> MAFSAGAESLLHQAREIQDEELRRFCSRVTKLLQEAPGPATVDALQRLFLIVSATKYPRRLEKMCVDLLQTTLCLPASPEQLQVLCAAILREMSPFNDLALSCDHTPNTRQLSLVASVLLAQGDRKGEIRCVSQRIFKILENRQPEGPSVRPLLPILSKVIGLAPGILMEDQTNLLSKRLVDWLRYASIQQGLPYSGGFFSTPRTRQPGPITEVDGAVASDFFTVLSTGQHFTEDQWVNMQAFSMLRKWLLHSGPEDPCSPDADDKSELEGSTLSVLSAASTASRLLPPRERLREVAFEYCQRLLEQSNRRALRKGDSDLQKACLVEAVSVLDVLCRQDPSFLYRTLSCLKALHRRLGEDPGSERALVPLAQFFLNHGEAAAMDAEAVYGQLLRGLPSERFHSPTLAFEVIHFCTHNLALFDSHFLSLLRLSFPSLFKFLAWNSPPLTAEFVVLLPALVDAGTAVEMLHALLDLPCLTAALDLQLRSTQTPSERLLWDISLRVPSCLEAFQDPQFQGLFRHLLRTKASGSTERLTPLHQVLKPMASCARVTQCAEAVPVLLQAFFSAVTQTADGALINQLALLLLERSDSLYPVPQYEARVHGVLSSQLLVLCKLKPSLVVELSRELLEFVGSVSSIHSRASVFTCVVWAIGEYLSVTWDKRCTAEQINKFFEALEALLFEVTQSRPLADLPCCPPEVVTALMTTLTKLASRSQDLIPRVSLFLSKMRTLAQNPATSSVHSEEGAESIRTRASELLTLLKMPSVAQFVFTPPAGVCQPRYHRDTNVALPLALRTVSRLVEKEAGLLPG;> MGPLSRDAWAQRLGAFRASPSAFMAGPEGEDLGRDLLSDLRSEKLSEQTKVSLLALSMEYPAQLWPDASAAEVAATSLLDTLVLLPPRPSALRRPLLLAATTALAAGGALGPTSGASCRLLPLLLGLAAGSDLGRGFVPASEQRPLQATACECLRELESCKPGLLGGSLGLLRGLLGQEGPVQPLSLLLALALRNTLVLQSRVGAGLGGLLTDKVSPTGGGPWDWTLVEEGDGRLQPQAPSWPAAEEGEGERSLTAREHSPEEARELRAAVIQLLDTSYLLTPVAQAQLLWLLGWALRGLQGQPPALFKPQLVRLLGTAQLTLLHAMLALKAAFGEALFTAQDEALLLRRLTLAAQHPA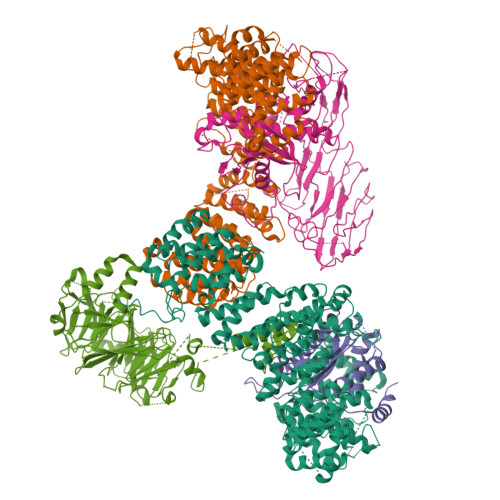LPPPTHLFYLHCVLSFPENWPLGPEGEEAAPLLLGPQLCRGLLPSLLHDPMALLARLHLLCLLCAEEEEEEKGQLPSPRHYLEELLAGLRQRAALDGGPRALATLCFQASYLVACCLAGQPTVLTPLIHGLAQLYQARPMLAPHFVDLLDQVDSELREPLKVVLRQVVVSRPGRDEALCWHLQMLAKVADGDAQSATLNFLQAAAAHCTNWDLQQGLLRVCRALLRAGVRGGLVDLLQVLARQLEDPDGRDHARLYYILLAHLAAPKLGVALGPSLAAPALASSLVAENQGFVAALMVQEAPALVRLSLGSHRVKGPLPVLKLQPEALEPIYSLELRFRVEGQLYAPLEAVHVPCLCPGRPARPLLLPLQPRCPAPARLDVHALYTTSTGLTCHAHLPPLFVNFADLFLPFPQPPEGAGLGFFEELWDSCLPEGAESRVWCPLGPQGLEGLVSRHLEPFVVVAQPPTSYCVAIHLPPDSKLLLRLEAALADGVPVALRTDDWAVLPLAGDYLRGLAAAV;> MVHAFLIHTLRAPNTEDTGLCRVLYSCVFGAEKSPDDPRPHGAERDRLLRKEQILAVARQVESMCRLQQQASGRPPMDLQPQSSDEQVPLHEAPRGAFRLAAENPFQEPRTVVWLGVLSLGFALVLDAHENLLLAEGTLRLLTRLLLDHLRLLAPSTSLLLRADRIEGILTRFLPHGQLLFLNDQFVQGLEKEFSAAWPR;> MAAEEGVASAASAGGSWGTAAMGRVLPMLLVPVPAEAMGQLGSRAQLRTQPEALGSLTAAGSLQVLSLTPGSRGGGRCCLEGPFWHFLWEDSRNSSTPTEKPKLLALGENYELLIYEFNLKDGRCDATILYSCSREALQKLIDDQDISISLLSLRILSFHNNTSLLFINKCVILHIIFPERDAAIRVLNCFTLPLPAQAVDMIIDTQLCRGILFVLSSLGWIYIFDVVDGTYVAHVDLALHKEDMCNEQQQEPAKISSFTSLKVSQDLDVAVIVSSSNSAVALNLNLYFRQHPGHLLCERILEDLPIQGPKGVDEDDPVNSAYNMKLAKFSFQIDRSWKAQLSSLNETIKNSKLEVSCCAPWFQDILHLESPESGNHSTSVQSWAFIPQDIMHGQYNVLQKDHAKTSDPGRSWKIMHISEQEEPIELKCVSVTGFTALFTWEVERMGYTITLWDLETQGMQCFSLGTKCIPVDSSGDQQLCFVLTENGLSLILFGLTQEEFLNRLMIHGSASTVDTLCHLNGWGR;> MALRAVWLIRHEPGTPLGGTVRFSRRYPTVEKRAKAFNGMTYVPVPEDGPFLRALLFQLRLLDDDKDFMERRDGCSRINKTSIYGLSVGGEELWPVIAFLRDSMIYASVPLVEQALSPRPPLISISGVSQGLELLLGIQDFLYSSQKNDTDLHTKLSQLPDLLLQACPLGTLLDANLQNSLNSINSVSVTQPQKQPAWKVGAYKGKAQISISITETVKCMQYGKQDIADTWQVAGTVACKCDLEGVMPAVTISLSLPTNGSPLQDIIVHPCVTSLDSAILTSSSIDTMDDSAFSGPYKFPFTPPLESFNLCHYTSQVPVPPILGSYHMKEEGVQLKVTVNFKLHESVRNNFEVCEAHIPFYNRGPITHLEYKASFGQLEVFREKSLLVWIIGQKFPKSMEISLSGTLTFGVKGHNKQPFDHICIGNTAYIKLNFRIADYTLTGCYADQHSVQVFASGKPKISAYRKLISSDYYIWNSKAPAPVTYASLLP Methyl 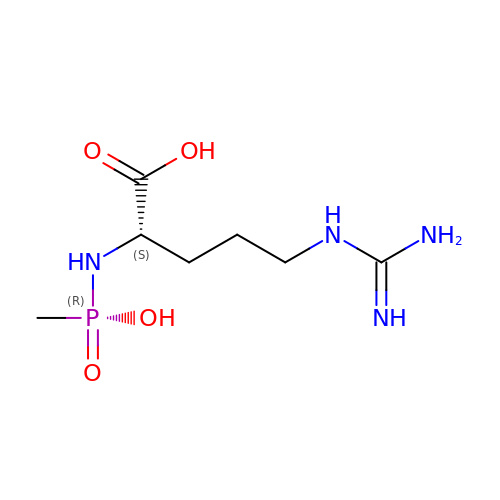phosphonated L-Arginine | C7 H17 N4 O4 P | BJBJPERGZRNAQZ-YFKPBYRVSA-N>GSNAGGSSPITGLVYDQRMMLHHNMWDSHHPELPQRISRIFSRHEELRLLSRCHRIPARLATEEELALCHSSKHISIIKSSEHMKPRDLNRLGDEYNSIFISNESYTCALLAAGSCFNSAQAILTGQVRNAVAIVRPPGHHAEKDTACGFCFFNTAALTARYAQSITRESLRVLIVDWDVHHGNGTQHIFEEDDSVLYISLHRYEDGAFFPNSEDANYDKVGLGKGRGYNVNIPWNGGKMGDPEYMAAFHHLVMPIAREFAPELVLVSAGFDAARGDPLGGFQVTPEGYAHLTHQLMSLAAGRVLIILEGGYNLTSISESMSMCTSMLLGDSPPSLDHLTPLKTSATVSINNVLRAHAPFWSSLR[2x]

The structure of HDAC6 stands out within the HDAC family due to the presence of two distinct functional catalytic domains (CD1 and CD2), both zinc-dependent and exhibiting differences in substrate preferences. Over the last few years, difluoromethyl-1,3,4-oxadiazole (DFMO) derivatives have emerged as a new promising class of highly selective, non-hydroxamic HDAC6 inhibitor. The inhibition mechanism involves the formation of a difluoroacetylhydrazide (DFAcH), which is generated in situ by the HDAC6-catalyzed hydrolysis of the DFMO warhead.

ITF7209, from our DFMO-focused medicinal chemistry program, was chosen as a new molecular model to further investigate the mechanism of action of this class of molecules. It should be noticed that this compound features a five-membered ring (thiophene) directly bound to the DFMO, a moiety that could induce different electronic effects on the ZBG and lead to a different binding geometry in the catalytic pocket, compared to the phenyl ring of ITF5924 (see section “X-Ray studies”). Moreover, the smaller cap-term of ITF7209 reduces the interaction with the binding site rim, which may minimize the potential impact of the ligand on the protein conformation. In this work, we report a new complex between zHDAC6-CD2 and the ITF7209 derivative, which is a novel DFMO displaying a previously unseen binding mode. The CHF2 moiety lies in the flat pocket mainly originated by Pro571, which is buried in a local interaction network between the fluorine atoms and the closest residues. Lastly, Tyr745 exhibits a possible halogen bond (d = 2.37 Å) with the fluorinated methyl substructure and a hydrogen bond (d = 2.51 Å) with N4. The comparison between the new structure of ITF7738 and that of compound 13 shows that the chemical nature of the “parent” DFMO does affect the binding mode of the resulting DFAcH. In turn, it is very possible that the specific conformation of the DFAcH-zHDAC6-CD2 complex dictates the relative prevalence of mechanism 1 or mechanism 2.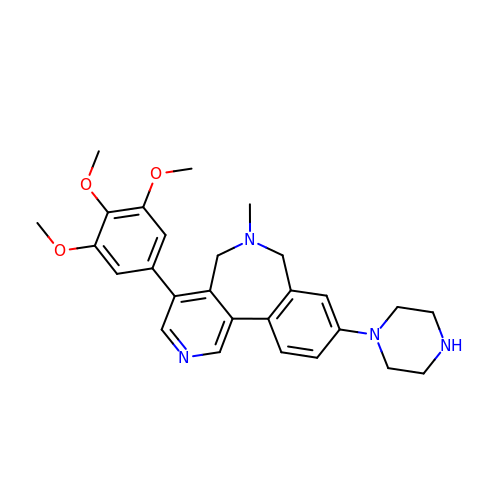6-methyl-9-piperazin-1-yl-4-(3,4,5-trimethoxyphenyl)-5,7-dihydropyrido[4,3-d][2]benzazepine | C27 H32 N4 O3 | YNAFROCLXSLUGD-UHFFFAOYSA-N WXG100 proteins are a group of proteins of approximately ∼100 residues in length that contain a conserved “Trp-Xaa-Gly (WXG)” motif. To investigate how specific sequence motifs translate into specific structural features, we determined the atomic structures of two representative complexes, the heterodimeric CFP-10/ESAT-6 complex and the homodimeric sagEsxA assembly. The overall structures of the two protein complexes are similar, with both forming a four-helix bundle, in which each monomer consists of a helix-loop-helix structural motif. However, the novelty of this contribution is that by using the iterative bio-informatics approach, we can show that the WXG100 protein superfamily can be divided into three subfamilies: CFP-10-, ESAT-6- and sagEsxA-like.

For example, the NMR structure of the CFP-10/ESAT-6 complex shows a heterodimeric four-helix bundle with flexible termini. More recently, we solved the X-ray structure of the same complex (CFP-10/ESAT-6). In contrast to the solution structure, the X-ray structure shows better ordered termini which adopt extended α-helical structures. In CFP-10, the WXG containing loop (residues 39–45) is three residues shorter than the corresponding loop of ESAT-6 (residues 39–48). In addition, it contains a 310-helix with hydrogen bonds originating only from main chain atoms, whereas, the loop of sagEsxA (residues 43–48) consists only of a single tight β-turn. The side chain of Y51 is located at the interface between the α1 and α2 helices of ESAT-6 where it forms an inter-helical hydrogen bond with the hydroxyl group of T37 and an intra-helical hydrogen bond with the side chain amide group of Q55. In particular, the indole ring of the conserved W43 is oriented towards two helices and together with Y51, W43 blocks the top interface of the helices α1 and α2. In addition, the WXG-motif of ESAT-6 forms an extended hydrogen-bonding network, where the main chain amine groups of W43-G44-G45 form hydrogen bonds to the main chain carbonyl groups of A40 and A41. In contrast, the WXG loop of ESAT-6 adopts a more rigid conformation due to the extensive hydrogen bond contacts. A FRET signal could only be detected in those samples where donor-CFP-10 was mixed with acceptor-ESAT-6 or vice versa. These results demonstrate that CFP-10 and ESAT-6 exclusively form heterodimer and that heterodimer formation is a spontaneous process.

>AMAEMKTDAATLAQEAGNFERISGDLKTQIDQVESTAGSLQGQWRGAAGTAAQAAVVRFQEAANKQKQELDEISTNIRQAGVQYSRADEEQQQALSSQMGF[2x];>[2x]TEQQWNFAGIEAAASAIQGNVTSIHSLLDEGKQSLTKLAAAWGGSGSEAYQGVQQKWDATATELNNALQNLARTISEAGQAMASTEGNVTGMFA>TRQFLIYNEDHKRCVDAVSPSAVQTAACNQDAESQKFRWVSESQIMSVAFKLCLGVPSKTDWVAITLYACDSKSEFQKWECKNDTLLGIKGEDLFFNYGNRQEKNIMLYKGSGLWSRWKIYGTTDNLCSRGYEAMYTLLGNANGATCAFPFKFENKWYADCTSAGRSDGWLWCGTTTDYDTDKLF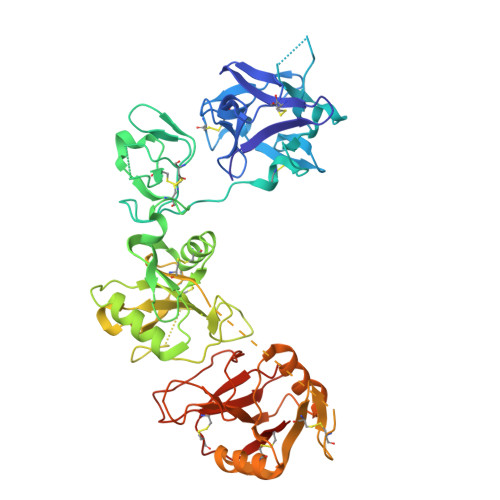GYCPLKFEGSESLWNKDPLTSVSYQINSKSALTWHQARKSCQQQNAELLSITEIHEQTYLTGLTSSLTSGLWIGLNSLSFNSGWQWSDRSPFRYLNWLPGSPSAEPGKSCVSLNPGKNAKWENLECVQKLGYICKKGNTTLNSFVIPSESDVPTHCPSQWWPYAGHCYKIHRDEKKIQRDALTTCRKEGGDLTSIHTIEELDFIISQLGYEPNDELWIGLNDIKIQMYFEWSDGTPVTFTKWLRGEPSHENNRQEDCVVMKGKDGYWADRGCEWPLGYICKMKSHHHHHH[2x]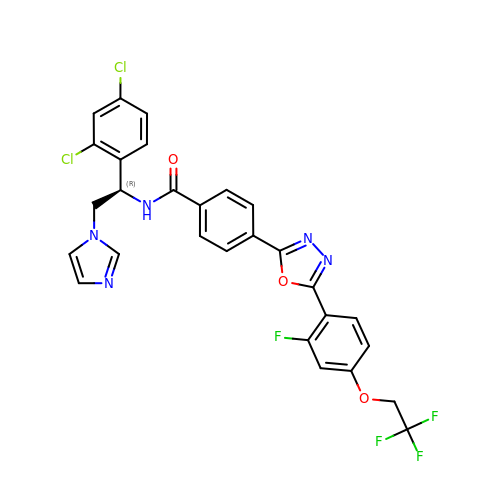N-[(1R)-1-(2,4-dichlorophenyl)-2-(1H-imidazol-1-yl)ethyl]-4-{5-[2-fluoro-4-(2,2,2-trifluoroethoxy)phenyl]-1,3,4-oxadiazol-2-yl}benzamide | C28 H19 Cl2 F4 N5 O3 | PFDAIZREODDAGQ-DEOSSOPVSA-N>MKPVTLYDVAEYAGVSYQTVSRV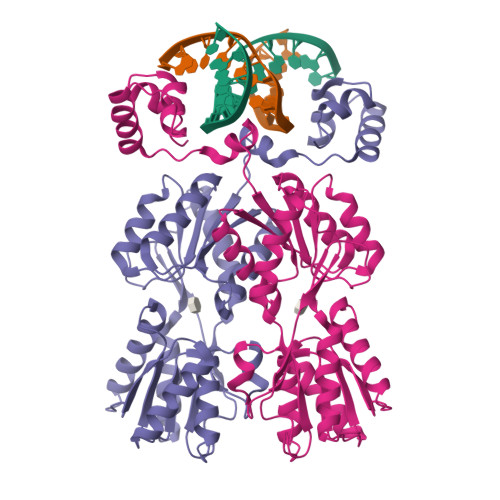VNQASHVSAKTREKVEAAMAELNYIPNRVAQQLAGKQSLLIGVATSSLALHAPSQIVAAIKSRADQLGASVVVSMVERSGVEACKTAVHNLLAQRVSGLIINYPLDDQDAIAVEAACTNVPALFLDVSDQTPINSIIFSHEDGTRLGVEHLVALGHQQIALLAGPLSSVSARLRLAGWHKYLTRNQIQPIAEREGDWSAMSGFQQTMQMLNEGIVPTAMLVANDQMALGAMRAITESGLRVGADISVVGYDDTEDSSCYIPPLTTIKQDFRLLGQTSVDRLLQLSQGQAVKGNQLLPVSLVKRKTTLAPN[3x]>[2x]MSIEKVPILGKETIHVGYGIADHIVREVIANLASSTYVIVTDTNMARTPQYSKLTDDFKTNLSEKRPESRLLTYCVSPGENNKNRATKAAVEDFLLQQGCTRDTVILAVGGGVIGDMIGFVAATFMRGVRVVQVPTTLLAMVDSSVGGKTAIDTPLGKNFIGAFHQPEYVF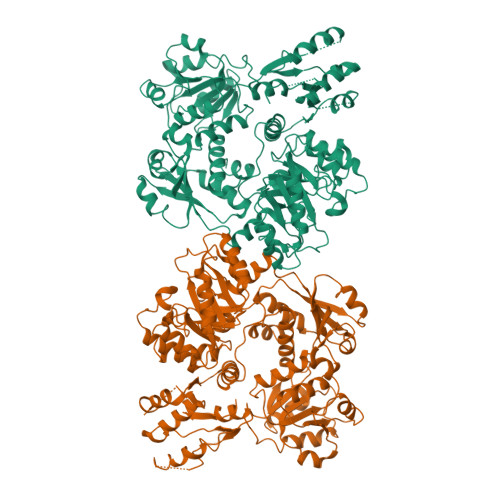CDVSFLETLPARQFINGMAEVVKTAAIWNEEEFTRLENFSKKFLSVVTSKKPDLQSIKAELVKTVLESVRVKAGVVSSDEKEAGLRNLLNFGHTIGHAIEAVLTPEALHGECVSIGMIKEAELSRYLGILPPVAVARLSKCLVAYGLPVSIDDKEFLKKVGPKRHYVEIDILLKKMAIDKKNDGSKIRCVLLEKIGKCYQLKAHQVSKQDLSFVLTDEVLVHPFTNPPKENIIVPPGSKSISNRALILAALGNGTVRVKNLLHSDDTKHMLDAVASLKGAEISTEDNGETIVVKGNGGNLVTSGEELYLGNAGTASRFLTTVASLVGKSQASDDVILTGNARMQERPIGPLVDALGSNGSEIEYLNKQGSLPLKISAGNGLKGGRIELAATISSQYVSSILMCAPYAKEPVTLALVGGKPISQLYIDMTCAMMKSFGIEVTKSTTEEYTYHIPKGTYKNPSEYVIESDASSATYPLAFAAMTGTSCTIPNIGSSSLQGDAKFAVDVLKPMGCKVEQTTTSTTVTGPPRGHLKPLPHVDMEPMTDAFLTASVVAAVAKGGSSTSITGIANQRVKECNRIEAMVTELAKFGVPANELPDGIEIHGIDIEDLKTPEISKRGVSSYDDHRVAMSFSLLAGLCKEPVLILERSTTGKTWPGWWDILHSKFKIELDGYEPPFNTDKHVDKSSDKSIIVIGMRGTGKSTLSEWLASFLGFKMLDMDKYLEEKLGTGIKSLIKAKGWEYFRQEEAIVAKECFTKFSKGYVLSTGGGIVEGEDARQQLKSYADNGGIVLHLHRDLDETVTFLAADTTRPAYSSEVQEVWLRREKWYHECSNYHFYSSHCSTEDEFNHLRRSFVNYIKLITGAERPVVPAGRSAAVVLTSPDLNEVVGDLESITIGADAVELRVDLFKDTSAEFVAAQIAVIRKHADLPIIYTVRTVSQGGKFPDENVDELKSLLLLGIRLGVAYVDLQLTAPNELIEEISSKKGFTRVIGTYQDINGELKWNNVEWKNKYNQGVSMNADIVRLVGKANSIQDNLDLENFKKQNTLKPLIAFNLGSQGKLSQVLNGTFTPISHKLLPNDEEFLTIGELNQTYFDIGGFTAKKFWVIGSPIEHSRSPNLHNAGYKALNLPYQFGRFEATDVDVVYDNLINKPDFGGLAITMPLKLDIMKFATKLSDAAETIGAVNTLIPIEGGYFGDNTDWVGISNSFIRAGVPPKSSSNGLVVGAGGTSRAAIYALHQMGCAKIYLVNRTAAKLEELVKSFPKDYNLEIVETEQQADKASKVSLAVSCIPADKPLDGEVLKKIERILSNGSEQSAGFKPTLLEASYKPRVTPIMKLTEEQYKWKVIPGVEMLVNQGDRQFKLHTGFTAPYEIIHRAVVEE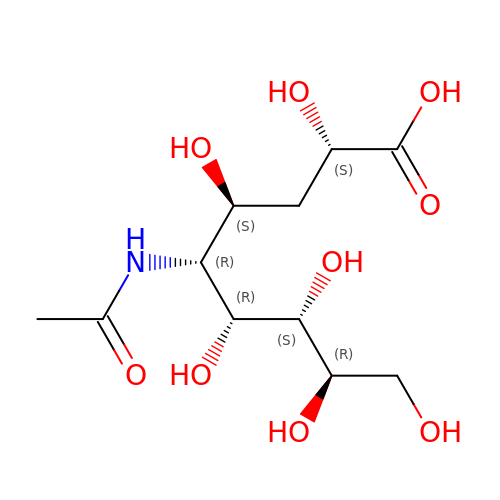(2~{S},4~{S},5~{R},6~{R},7~{S},8~{R})-5-acetamido-2,4,6,7,8,9-hexakis(oxidanyl)nonanoic acid | C11 H21 N O9 | REORMAHRVILHOU-HQBQHRAMSA-N>[2x]SNAMTQLTREQVLELFHQRSSTRYYDPTKKISDEDFECILE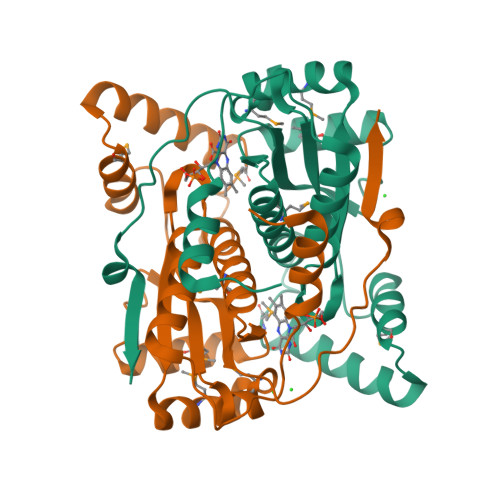CGRLSPSSVGSEPWKFLVIQNKTLREKMKPFSWGMINQLDNCSHLVVILAKKNARYDSPFFVDVMARKGLNAEQQQAALTKYKALQEEDMKLLENDRTLFDWCSKQTYIALANMLTGASALGIDSCPIEGFHYDKMNECLAEEGLFDPQEYAVSVAATFGYRSRDIAKKSRKGLDEVVKWVG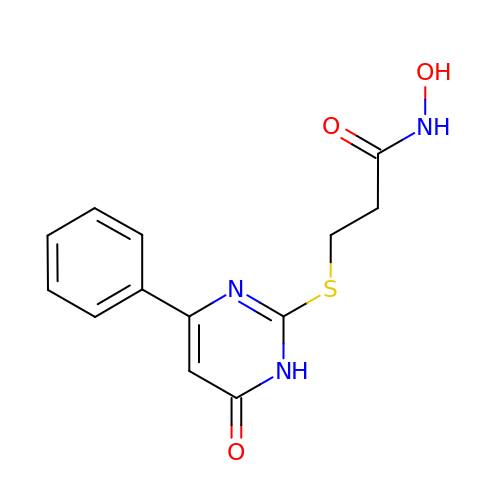N-hydroxy-3-[(6-oxo-4-phenyl-1,6-dihydropyrimidin-2-yl)sulfanyl]propanamide | C13 H13 N3 O3 S | WNPFBIDOQFZHQF-UHFFFAOYSA-N> KEYDIYVSYARNAEEEEFVLLTLRGVLENEFGYKLCIFDRDSLPGGNTVEAVFDFIQRSRRMIVVLSPDYVTEKSISMLEFKLGVMCQNSIATKLIVVEYRPLEHPHPGILQLKES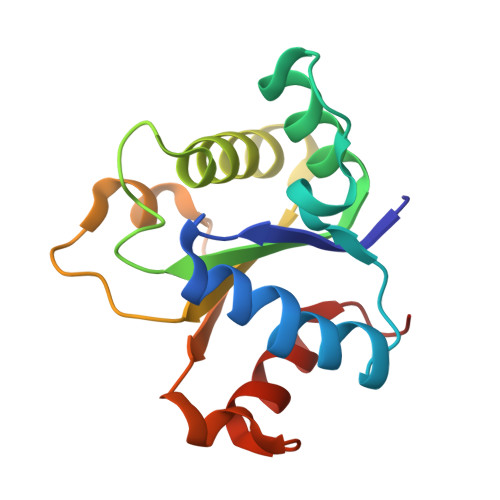VSFVSWKGEKSKHSGSKFWKALRLALPLRS> MKILVIGAGPAGLVFASQLKQARPLWAIDIVEKNDEQEVLGWGVVLPGRPGQHPANPLSYLDAPERLNPQFLEDFKLVHHNEPSLMSTGVLLCGVERRGLVHALRDKCRSQGIAIRFESPLLEHGELPLADYDLVVLANGV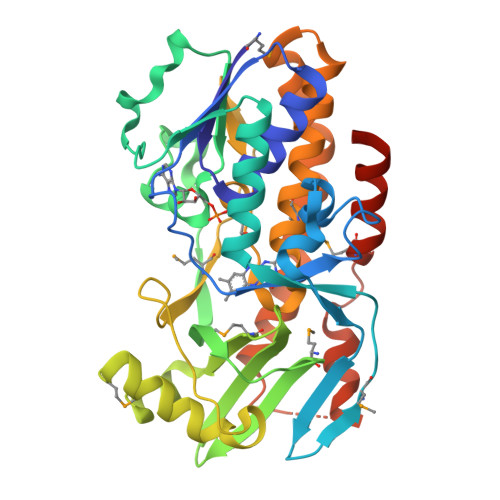NHKTAHFTEALVPQVDYGRNKYIWYGTSQLFDQMNLVFRTHGKDIFIAHAYKYSDTMSTFIVECSEETYARARLGEMSEEASAEYVAKVFQAELGGHGLVSQPGLGWRNFMTLSHDRCHDGKLVLLGDALQSGHFSIGHGTTMAVVVAQLLVKALCTEDGVPAALKRFEERALPLVQLFRGHADNSRVWFETVEERMHLSSAEFVQSFDARRKSLPPMPEALAQNLRYALQRLEHHHHHH> KPKLLNKFDKTIKAELDAAEKLRKRGKIEEAVNAFKELVRKYPQSPRARYGKAQCEDDLAEKRRSNEVLRGAIETYQEVASLPDVPADLLKLSLKRRSDRQQFLGHMRGSLLTLQRLVQLFPNDTSLKNDLGVGYLLIGDNDNAKKVYEEVLSVTPNDGFAKVHYGFILKAQNKIAESIPYLKEGIESGDPGTDDGRFYFHLGDAMQRVGNKEAYKWYELGHKRGHFASVWQRSLYNVNGLKAQPWWTPKETGYTELVKSLERNWKLIRDEGLAVMDKAKGLFLPEDENLREKGDWSQFTLWQQGRRNENACKGAPKTCTLLEKFPETTGCRRGQIKYSIMHPGTHVWPHTGPTNCRLRMHLGLVIPKEGCKIRCANETKTWEEGKVLIFDDSFEHEVWQDASSFRLIFIVDVW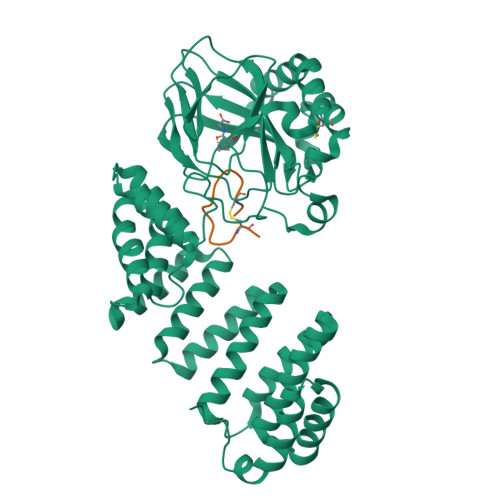HPELTPQQRRSLPAI;> DGDQCETSPCQNQGKCKDGLGEYTCT>MDALELLINRRSASRLAEPAPTGEQLQNILRAGMRAPDHKSMQPWHFFVIEGEGRERFSAVLEQGAIAAGSDDKAIDKARNAPFRAPLIITVVAKCEENHKVPRWEQEMSAGCAVMAMQMAAVAQGFGGIWRSGALTESPVVREAFG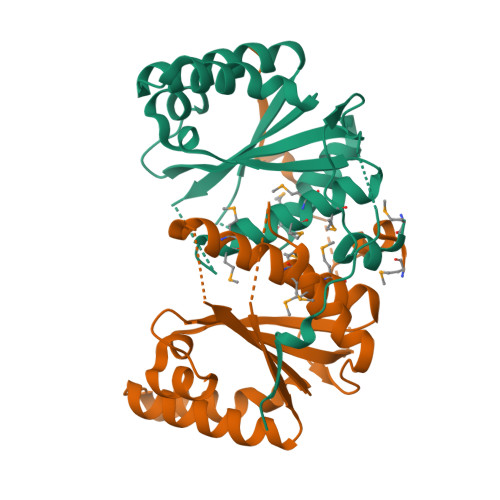CREQDKIVGFLYLGTPQLKASTSINVPDPTPFVTYFHH[2x]>[2x]MGSSHHHHHHSSGLEVLFQGPAMATKKVHIISHSHWDREWYMAYEQHHMRLINLIDDLLEVFQTDPDFHSFHLDGQTIILDDYLKVRPEREPEIRQAIASGKLRIGPFYILQDDFLTSSESNVRNMLIGKEDCDRWGASVPLGYFPDTFGNMGQTPQLMLKAGLQAAAFGRGIRPTGFNNQVDTSEKYSSQFSEISWQGPDNSRILGLLFANWYSNGNEIPTTEAEARLFWDKKLADAERFASTKHLLMMNGCDHQPVQLDVTKAIALANQLYPDYEFVHSCFEDYLADLADDLPENLSTVQGEITSQETDGWYTLANTASARIYLKQANTRVSRQLENITEPLAAMAYEVTSTYPHDQLRYAWKTLMQNHPHDSICGCSVDSVHREMMTRFEKAYEVGHYLAKEAAKQIADAIDTRDFPMDSQPFVLFNTSGHSKTSVAELSLTWKKYHFGQRFPKEVYQEAQEYLARLSQSFQIIDTSGQVRPEAEILGTSIAFDYDLPKRSFREPYFAIKVRLRLPITLPAMSWKTLALKLGNETTPSETVSLYDDSNQCLENGFLKVMIQTDGRLTITDKQSGLIYQDLLRFEDCGDIGNEYISRQPNHDQPFYADQGTIKLNIISNTAQVAELEIQQTFAIPISADKLLQAEMEAVIDITERQARRSQEKAELTLTTLIRMEKNNPRLQFTTRFDNQMTNHRLRVLFPTHLKTDHHLADSIFETVKRPNHPDATFWKNPSNPQHQECFVSLFDGENGVTIGNYGLNEYEILPDTNTIAITLLRSVGEMGDWGYFPTPEAQCLGKHSLSYSFESITKQTQFASYWRAQEGQVPVITTQTNQHEGTLAAEYSYLTGTNDQVALTAFKRRLADNALITRSYNLSNDKTCDFSLSLPNYNAKVTNLLEKDSKQSTPSQLGKAEILTLAWKKQ

Streptococcus pyogenes M1 GAS SF370 ORF Spy1604 encodes a putative GH38 α-mannosidase. We have shown that The S. pyogenes ORF spy1604 encodes an α−1,3 mannosidase that is active on disaccharides, some aryl glycosides and can also effectively deglycosylate human N-glycans in vitro. This, coupled to the presence of a gene encoding an N-acetyl glucosaminidase (Spy1600) on the operon (an enzyme known to break β−linked N-acetylglucosaminides) would suggest a role, in vivo, in the utilization of human glycan-derived carbohydrates as a nutrient source. Comparison of SpGH38 with Drosophila Golgi α−mannosidase II suggests a conserved domain architecture and catalytic centre in which diversification in the “leaving group” subsites accounts for the subtly different specificity.

Here we report, what we believe to be, the first structure of a bacterial α−mannosidase from the human pathogen S. pyogenes bound to the therapeutically important inhibitor swainsonine. The natural product swainsonine is known to be a versatile glycosidase inhibitor having previously been used to study the active center of the Drosophila enzyme. In addition to the favorable electrostatic interactions discussed previously, the position of F127 is conserved across α-mannosidase II active centers. Additionally, swainsonine is stabilized through stacking interactions of W18 with the five-membered ring, suggesting that the two aromatic residues contribute to positioning mannose into the correct orientation in the −1 subsite. Other conserved active centre residues, D125 and D232 are in equivalent positions to the catalytic nucleophile and general acid/base, respectively, of dGMII. As with the Drosophila enzyme, it is likely that R149 will encourage D125 to be ionized (as required for a nucleophile). The hydrogen-bond from Y192 to D125 may also stabilize the ionized form of D125. D232 will likely be neutral due to negative charge repulsion from D125, as expected for the acid/base. The structure of SpGH38 is consistent with previous proposals (notably) concerning the chemical basis for catalysis with net retention of anomeric configuration in this family.N-[(E)-3-[(2R,3S,4R,5R)-3,4-dihydroxy-5-(4-oxopyridin-1-yl)oxolan-2-yl]prop-2-enyl]-2,3-dihydroxy-5-nitro-benzamide | C19 H19 N3 O9 | 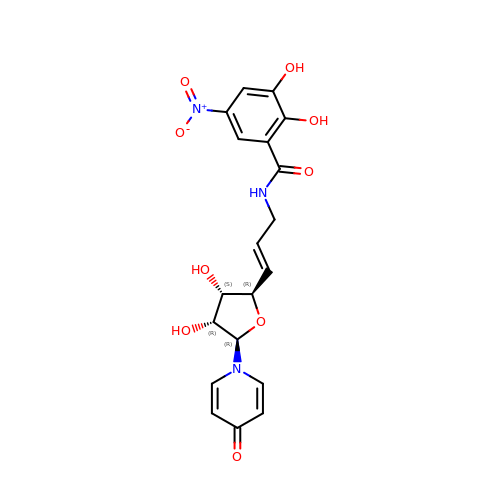HVTOTCCLXQPREB-LDNIWRHMSA-N> GSKKRQRFVDKNGRCNVQHGNLGSERAETLMFSEHAVISMRDGKLTLMFRVGNLRNSH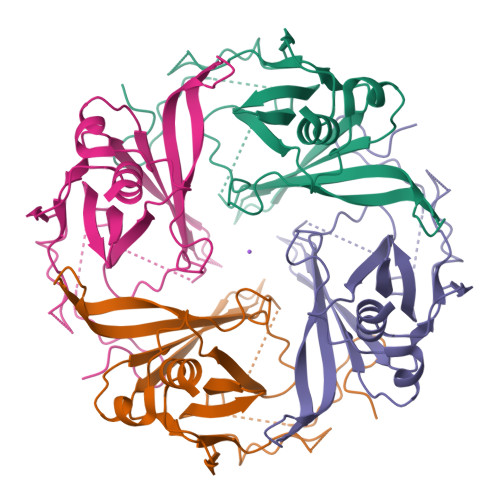MVEAQIRCKLLKSRQTPEGEFLPLDQLELDVGFSTGADQLFLVSPLTICHVIDAKSPFYDLSQRSMQTEQFEVVVILEGIVETTGMTCQARTSYTEDEVLWGHRFFPVISLEEGFFKVDYSQFHATFEVPTPPYSVKEQEEMLLMSSPL>[2x]MALSAEGSSGGSRGGSPKAEAASVPSWPQILGRLTDNRD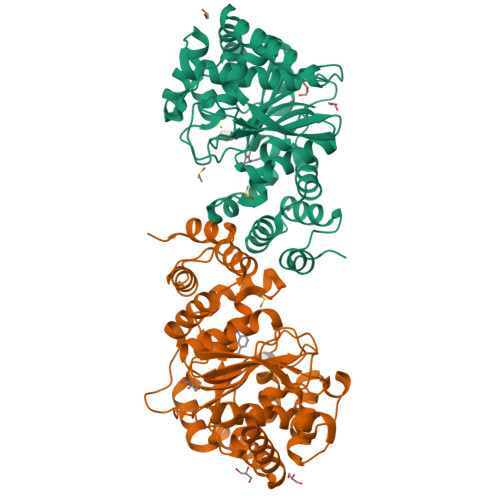LARGQAAWAMDQIMTGNARPAQIAAFAVAMTMKAPTADEVGELAGVMLSHAHPLPADTVPDDAVDVVGTGGDGVNTVNLSTMAAIVVAAAGVPVVKHGNRAASSLSGGADTLEALGVRIDLGPDLVARSLAEVGIGFCFAPRFHPSYRHAAAVRREIGVPTVFNLLGPLTNPARPRAGLIGCAFADLAEVMAGVFAARRSSVLVVHGDDGLDELTTTTTSTIWRVAAGSVDKLTFDPAGFGFARAQLDQLAGGDAQANAAAVRAVLGGARGPVRDAVVLNAAGAIVAHAGLSSRAEWLPAWEEGLRRASAAIDTGAAEQLLARWVRFGRQILEHHHHHH>[2x]MRGSHHHHHHGSMPVAGSELPRRPLPPAAQERDAEPRPPHGELQYLGQIQHILRCGVRKDDRTGTGTLSVFGMQARYSLRDEFPLLTTKRVFWKGVLEELLWFIKGSTNAKELSSKGVKIWDANGSRDFLDSLGFSTREEGDLGPVYGF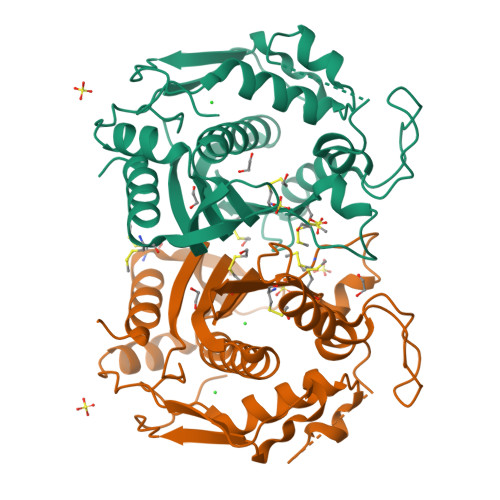QWRHFGAEYRDMESDYSGQGVDQLQRVIDTIKTNPDDRRIIMCAWNPRDLPLMALPPCHALCQFCVVNSELSCQLYQRSGDMGLGVPFNIASYALLTYMIAHITGLKPGDFIHTLGDAHIYLNHIEPLKIQLQREPRPFPKLRILRKVEKIDDFKAEDFQIEGYNPHPTIKMEMAV>[2x]AHMFERVKTFQVPSPSIGTLPPAPDFKNDINEQLPDKTNPVITHFSTIPYIMANDATFNSHQQIQYSPYYKLVRIQYWEKVTQRILGPRDDYEYNKTKGISKTDQVSMTETVSMSVGADFGFMFKGFSASLSAQITKELSVTKSTSTTEMTEETYKEKYTNPFNYELARAQYMLVNEFYVTRMDGTRITANWTLRDNTQTVTRIFPKS

Cry78Aa is a novel protein identified from the Bt C9F1 strain that effectively kills rice planthoppers, with median lethal concentration (LC50) values against Laodelphax striatellus and Nilaparvata lugens of 6.89 and 15.78 μg ml−1, respectively. Here, we report the crystal structure of Cry78Aa, which consists of two domains: a C-terminal β-pore forming domain belonging to the aerolysin family and an N-terminal trefoil domain resembling the S-type ricin B lectin. We also found that Cry78Aa binds carbohydrates such as galactose derivatives and is essential for insecticidal activity against Laodelphax striatellus. Bioassays showed that the NTD or CTD of Cry78Aa alone has no toxicity against planthopper nymphs, indicating that its insecticidal activity is dependent on the cooperation of both domains.

We also resolved the structure of Cry78Aa155-359, which resembles the solitary pore-forming domain, and found that it has an identical conformation with Cry78Aa13-359. After growing and optimizing the selenomethionine derivative crystal of Cry78Aa155-359, its structure was determined by the SAD method and refined to 2.4 Å resolution with Rwork and Rfree values of 0.198 and 0.249, respectively. Cry78Aa155-359 packed as a dimer in the crystal, and its two protomers were almost superimposed on each other. Structural alignment of Cry78Aa13-359 (Mol A) and Cry78Aa155-359 (Mol B) revealed nearly identical conformations, with a root-mean-square deviation (RMSD) of 0.566 Å over 175 Cα atoms. The structure of Cry78Aa155-359 represents the conformation of the CTD in the absence of the NTD and has a domain organization similar to that in Cry78Aa13-359. According to the structure of BinA/B, which has significant structural similarity with Cry78Aa, the CTD of Cry78Aa can be further divided into the sheet domain, TM domain and sandwich domain. Structural comparison of Cry78Aa13-359 and Cry78Aa155-359 indicated that the β-pore-forming domain in the presence or absence of the NTD was nearly superimposed, suggesting that the absence of the NTD of Cry78Aa did not result in a dramatic conformational change in the CTD pore-forming domain. Similar results were observed when testing the effects of the pore-forming domain Cry78Aa155-359 on the survival of the nymphs: nearly all the nymphs in the assay remained alive under the same conditions. Cry78Aa155-359 had an apparent MW of 23.7 kDa, which was in accordance with its monomeric state of Cry78Aa155-359 (23.7 kDa). However, Cry78Aa155-359 has several characteristic features of aerolysin-type pore-forming toxins. Sequence analysis showed that 20.5% of Cry78Aa155-359 consisted of either serine (7.8%) or threonine (12.7%).>MNPERSERIEIPVLPLRDVVVYPHMVIPLFVGREKSIRCLEAAMDHDKKIMLVAQKEASTDEPGVNDLFTVGTVASILQMLKLPDGTVKVLVEGLQRARISALSDNGEHFSAKAEYLESPTIDEREQEVLVRTAISQFEGYIKLNKKIPPEVLTSLNSIDDPARLADTIAAHMPLKLADKQSVLEMSDVNERLEYLMAMMESEIDLLQVEKRIRNRVKKQMEKSQREYYLNEQMKAIQKELGEMDDAPDENEALKRKIDAAKMPKEAKEKAEAELQKLKMMSPMSAEATVVRGYIDWMVQVPWNARSKVKKDLRQAQEILDTDHYGLERVKDRILEYLAVQSRVNKIKGPILCLVGPPGVGKTSLGQSIAKATGRKYVRMALGGVRDEAEIRGHRRTYIGSMPGKLIQKMAKVGVKNPLFLLDEIDKMSSDMRGDPASALLEVLDPEQNVAFSDHYLEVDYDLSDVMFVATSNSMNIPAPLLDRMEVIRLSGYTEDEKLNIAKRHLLPKQIERNALKKGELTVDDSAIIGIIRYYTREAGVRGLEREISKLCRKAVKQLLLDKSLKHIEINGDNLHDYLGVQRFDYGRADNENRVGQVTGLAWTEVGGDLLTIETACVPGKGKLTYTGSLGEVMQESIQ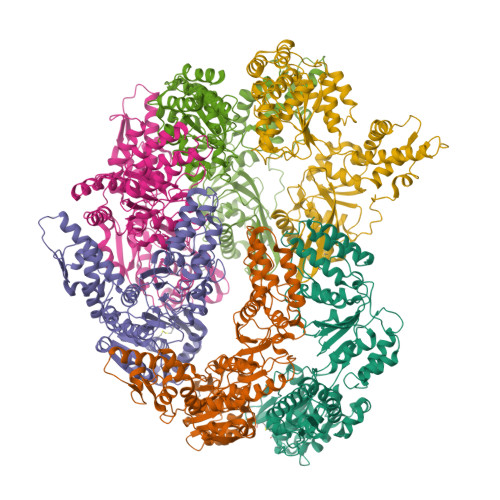AALTVVRARAEKLGINPDFYEKRDIHVHVPEGATPKDGPAAGIAMCTALVSCLTGNPVRADVAMTGEITLRGQVLPIGGLKEKLLAAHRGGIKTVLIPFENKRDLEEIPDNVIADLDIHPVKRIEEVLTLALQNEPSGMQVVTAK[6x]> LERRTFGSYKIEELTIRNDQPTRNTNLSLSQSTENRLSTKKIPLLDDGIFELLNYLIDGTNFNKTCYCGFNYSHLPNLERDFNIASLYVRENFEICTDQLDLANYVRQPNISIKSPDFTVCLEYVLKTVVESESSTKDQKDDESQKPTSTDSTKNEQETKFVEMSLLPLLNRESEESLTEEILEGEGAVVNVLKLFIKGFLMHLGENPNSYDRQLTVEKYRPLLVS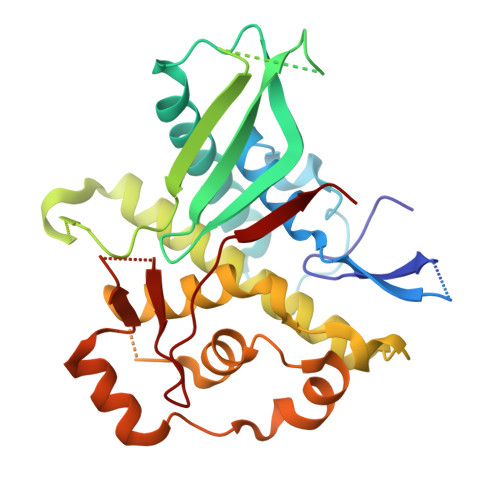IVGYEYLVGTTVPEKKINHIYYQLATFDNYPFDLLRFQLSSLISTPTSILERITKEGLFKIITSSTLRGAPRQTVLFRGINGSESFLNIKRYRRF>[6x]AMNNTIINSLIGGDDSIKRSNVFAVDSQIPTLYMPQYISLSGVMTNDGPDNQAIASFEIRDQYITALNHLVLSLELPEVKGMGRFGYVPYVGYKCINHVSISSCNGVIWEIEGEELYNNCINNTIALKHSGYSSELNDISIGLTPNDTIKEPSTVYVYIKTPFDVEDTFSSLKLSDSKITVTVTFNPVSDIVIRDSSFDFETFNKEFVYVPELSFIGYMVKNVQIKPSFIEKPRRVIGQINQPTATVTEVHAATSLSVYTKPYYGNTDNKFISYPGYSQDEKDYIDAYVSRLLDDLVIVSDGPPTGYPESAEIVEVPEDGIVSIQDADVYVKIDNVPDNMSVYLHTNLLMFGTRKNSFIYNISKKFSAITGTYSDATKRTIFAHISHSINIIDTSIPVSLWTSQRNVYNGDNRSAESKAKDLFINDPFIKGIDFKNKTDIISRLEVRFGNDVLYSENGPISRIYNELLTKSNNGTRTLTFNFTPK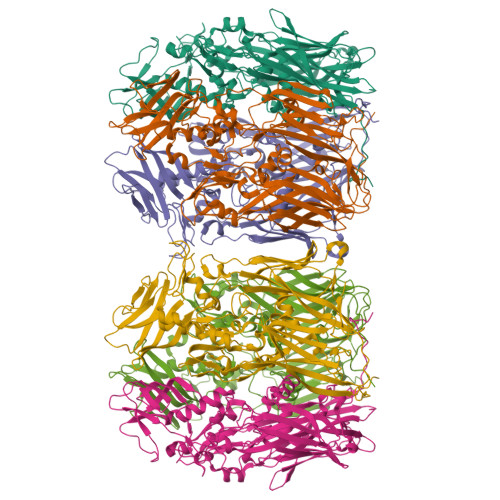IFFRPTTITANVSRGKDKLSVRVVYSTMDVNHPIYYVQKQLVVVCNDLYKVSYDQGVSITKIMG> MGSDKIHHHHHHMKLLKIYLGEKDKHSGKPLFEYLVKRAYELGMKGVTVYRGIMGFGHKRHMHR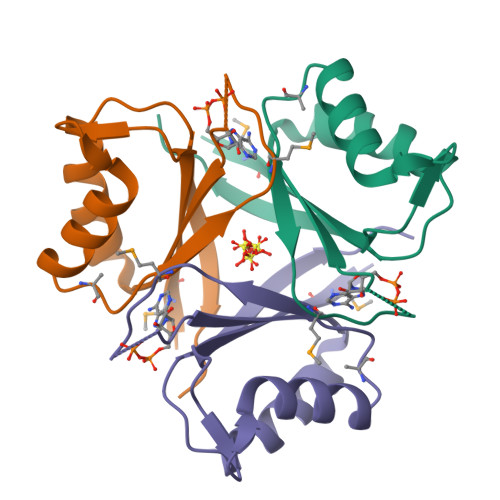SDFFSLSPDLPIVLEIVDEEERINLFLKEIDNIDFDGLVFTADVNVVKMG> MAYKPQFYPGATKIAQNRRDHLNPDFELEKLREIPDEELVKVMGHRQPGEDYKTVHPPLEEMDLPEDYVRDLVEPISGAKEGHRIRYIQFADSMYFAPAQPYDRARMYMWRFRGVDTGSLSGRQVIEMRESNLEEISKNVLMDTSL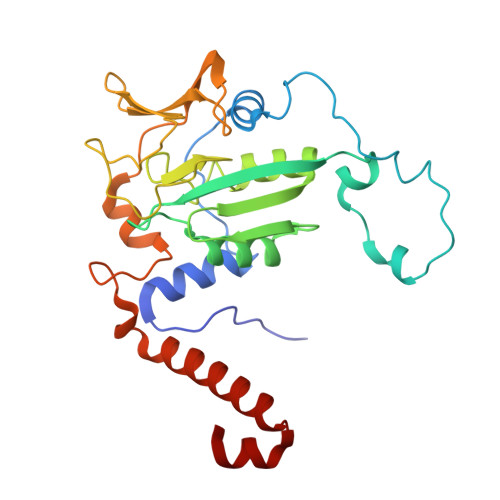FDPARIGMRGATVHGHSLRLDENGLMFDALQRYVYDEKTGHVVYVKDQVGRPLDEPVDVGEPLPEEKLREITTIYRKDGVPMRDDEELLTVVKRIHRARTLGGYMPVNEVFDKLL>GSHGMGGVDFEGFRKLQRADGFASILAIGTANPPNAVDQSTYPDFYFRITGNEHNTELKDKFKRICERSAIKQRYMYLTEEILKKNPDVCAFVEVPSLDARQAMLAMEVPRLAKEAAEKAIQEWGQSKSGITHLIFCSTTTPDLPGADFEVAKLLGLHPSVKRVGVFQHGCFAGGTVLRMAKDLAENNRGARVLVICSETTAVTFRGPSETHLDSLVGQALFGDGASALIVGADPIPQVEKACFEIVWTAQTVVPNSEGAIGGKVREVGLTF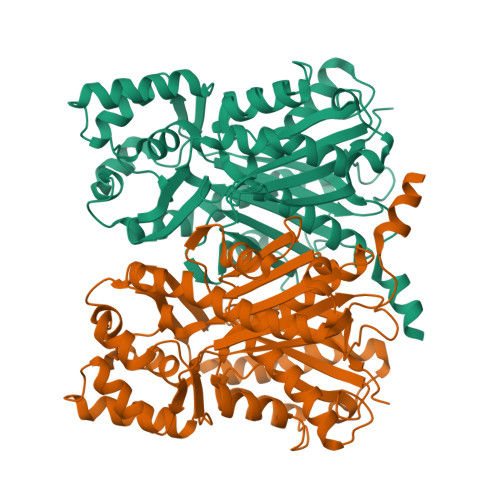QLKGAVPDLISANIENCMVEAFSQFKISDWNKLFWVVHPGGRAILDRVEAKLNLDPTKLIPTRHVMSEYGNMSSACVHFILDQTRKASLQNGCSTTGEGLEMGVLFGFGPGLTIETVVLKSVPIQ[6x]>MQGSVTEFLKPRLVDIEQVSSTHAKVTLEPLERGFGHTLGNALRRILLSSMPGCAVTEVEIDGVLHEYSTKEGVQEDILEILLNLKGLAVRVQGKDEVILTLNKSGIGPVTAADITHDGDVEIVKPQHVICHLTDENASISMRIKVQRGRGYVPASTRIHSEEDERPIGRLLVDACYSPVERIAYNVEAARVEQRTDLDKLVIEMETNGTIDPEEAIRRAATILAEQLEAFVDLRDVRQPEVKEEKPEFDPILLRPVDDLELTVRSANCLKAEAIHYIGDLVQRTEVELLKTPNLGKKSLTEIKDVLASRGLSLGMRLENWPPASIADE[2x];> MVYSYTEKKRIRKDFGKRPQVLDVPYLLSIQLDSFQKFIEQDPEGQYGLEAAFRSVFPIQSYSGNSELQYVSYRLGEPVFDVQECQIRGVTYSAPLRVKLRLVIYEREAPEGTVKDIKEQEVYMGEIPLMTDNGTFVINGTERVIVSQLHRSPGVFFDSDKGKTHSSGKVLYNARIIPYRGSWLDFEFDPKDNLFVRIDRRRKLPATIILRALNYTTEQILDLFFEKVIFEIRDNKLQMELVPERLRGETASFDIEANGKVYVEKGRRITARHIRQLEKDDVKLIEVPVEYIAGKVVAKDYIDESTGELICAANMELSLDLLAKLSQSGHKRIETLFTNDLDHGPYISETLRVDPTNDRLSALVEIYRMMRPGEPPTREAAESLFENLFFSEDRYDLSAVGRMKFNRSLLREEIEGSGILSKDDIIDVMKKLIDIRNGKGEVDDIDHLGNRRIRSVGEMAENQFRVGLVRVERAVKERLSLGDLDTLMPQDMINAKPISAAVKEFFGSSQLSQFMDQNNPLSEITHKRRISALGPGGLTRERAGFEVRDVHPTHYGRVCPIETPEGPNIGLINSLSVYAQTNEYGFLETPYRKVTDGVVTDEIHYLSAIEEGNYVIAQANSNLDEEGHFVEDLVTCRSKGESSLFSRDQVDYMDVSTQQVVSVGASLIPFLEHDDANRALMGANMQRQAVPTLRADKPLVGTGMERAVAVDSGVTAVAKRGGVVQYVDASRIVIKVNEDEMYPGEAGIDIYNLTKYTRSNQNTCINQMPCVSLGEPVERGDVLADGPSTDLGELALGQNMRVAFMPWNGYNFEDSILVSERVVQEDRFTTIHIQELACVSRDTKLGPEEITADIPNVGEAALSKLDESGIVYIGAEVTGGDILVGKVTPKGETQLTPEEKLLRAIFGEKASDVKDSSLRVPNGVSGTVIDVQVFTRDGVEKDKRALEIEEMQLKQAKKDLSEELQILEAGLFSRIRAVLVAGGVEAEKLDKLPRDRWLELGLTDEEKQNQLEQLAEQYDELKHEFEKKLEAKRRKITQGDDLAPGVLKIVKVYLAVKRRIQPGDKMAGRHGNKGVISKINPIEDMPYDENGTPVDIVLNPLGVPSRMNIGQILETHLGMAAKGIGDKINAMLKQQQEVAKLREFIQRAYDLGADVRQKVDLSTFSDEEVMRLAENLRKGMPIATPVFDGAKEAEIKELLKLGDLPTSGQIRLYDGRTGEQFERPVTVGYMYMLKLNHLVDDKMHARSTGSYSLVTQQPLGGKAQFGGQRFGEMEVWALEAYGAAYTLQEMLTVKSDDVNGRTKMYKNIVDGNHQMEPGMPESFNVLLKEIRSLGINIELEDE;> MKDLLKFLKAQTKTEEFDAIKIALASPDMIRSWSFGEVKKPETINYRTFKPERDGLFCARIFGPVKDYECLCGKYKRLKHRGVICEKCGVEVTQTKVRRERMGHIELASPTAHIWFLKSLPSRIGLLLDMPLRDIERVLYFESYVVIEGGMTNLERQQILTEEQYLDALEEFGDEFDAKMGAEAIQALLKSMDLEQECEQLREELNETNSETKRKKLTKRIKLLEAFVQSGNKPEWMILTVLPVLPPDLRPLVPLDGGRFATSDLNDLYRRVINRNNRLKRLLDLAAPDIIVRNEKRMLQEAVDALLDNGRRGRAITGSNKRPLKSLADMIKGKQGRFRQNLLGKRVDYSGRSVITVGPYLRLHQCGLPKKMALELFKPFIYGKLELRGLATTIKAAKKMVEREEAVVWDILDEVIREHPVLLNRAPTLHRLGIQAFEPVLIEGKAIQLHPLVCAAYNADFDGDQMAVHVPLTLEAQLEARALMMSTNNILSPANGEPI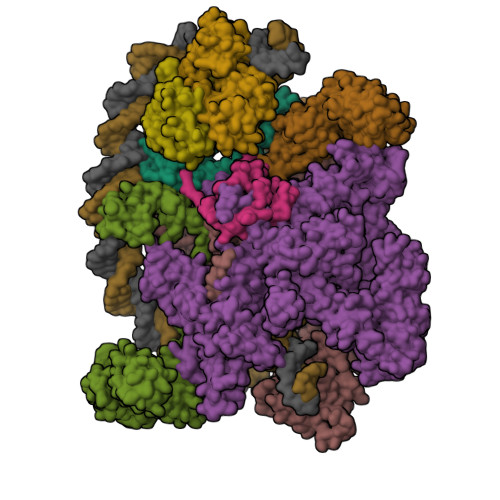IVPSQDVVLGLYYMTRDCVNAKGEGMVLTGPKEAERLYRSGLASLHARVKVRITEYEKDANGELVAKTSLKDTTVGRAILWMIVPKGLPYSIVNQALGKKAISKMLNTCYRILGLKPTVIFADQIMYTGFAYAARSGASVGIDDMVIPEKKHEIISEAEAEVAEIQEQFQSGLVTAGERYNKVIDIWAAANDRVSKAMMDNLQTETVINRDGQEEKQVSFNSIYMMADSGARGSAAQIRQLAGMRGLMAKPDGSIIETPITANFREGLNVLQYFISTHGARKGLADTALKTANSGYLTRRLVDVAQDLVVTEDDCGTHEGIMMTPVIEGGDVKEPLRDRVLGRVTAEDVLKPGTADILVPRNTLLHEQWCDLLEENSVDAVKVRSVVSCDTDFGVCAHCYGRDLARGHIINKGEAIGVIAAQSIGEPGTQLTMRTFHIGGAASRAAAESSIQVKNKGSIKLSNVKSVVNSSGKLVITSRNTELKLIDEFGRTKESYKVPYGAVLAKGDGEQVAGGETVANWDPHTMPVITEVSGFVRFTDMIDGQTITRQTDELTGLSSLVVLDSAERTAGGKDLRPALKIVDAQGNDVLIPGTDMPAQYFLPGKAIVQLEDGVQISSGDTLARIPQESGGTKDITGGLPRVADLFEARRPKEPAILAEISGIVSFGKETKGKRRLVITPVDGSDPYEEMIPKWRQLNVFEGERVERGDVISDGPEAPHDILRLRGVHAVTRYIVNEVQDVYRLQGVKINDKHIEVIVRQMLRKATIVNAGSSDFLEGEQVEYSRVKIANRELEANGKVGATYSRDLLGITKASLATESFISAASFQETTRVLTEAAVAGKRDELRGLKENVIVGRLIPAGTGYAYHQDRMRRRAAGEAPAAPQVTAEDASASLAELLNAGLGGSDNEHHHHHH;> ARVTVQDAVEKIGNRFDLVLVAARRARQMQVGGKDPLVPEENDKTTVIALREIEEGLINNQILDVRERQEQQEQEAAELQAVTAIAEGRR;> MEQNPQSQLKLLVTRGKEQGYLTYAEVNDHLPEDIVDSDQIEDIIQMINDMGIQVMEEAPDADDLMLAENTADEDAAEAAAQVLSSVESEIGRTTDPVRMYMREMGTVELLTREGEIDIAKRIEDGINQVQCSVAEYPEAITYLLEQYNRVEAEEARLSDLITGFVDPNAEEDLAPTATHVGSELSQEDLDDDEDEDEEDGDDDSADDDNSIDPELAREKFAELRAQYVVTRDTIKAKGRSHATAQEEILKLSEVFKQFRLVPKQFDYLVNSMRVMMDRVRTQERLIMKLCVEQCKMPKKNFITLFTGNETSDTWFNAAIAMNKPWSEKLHDVSEEVHRALQKLQQIEEETGLTIEQVKDINRRMSIGEAKARRAKKEMVEANLRLVISIAKKYTNRGLQFLDLIQEGNIGLMKAVDKFEYRRGYKFSTYATWWIRQAITRSIADQARTIRIPVHMIETINKLNRISRQMLQEMGREPTPEELAERMLMPEDKIRKVLKIAKEPISMETPIGDDEDSHLGDFIEDTTLELPLDSATTESLRAATHDVLAGLTAREAKVLRMRFGIDMNTDHTLEEVGKQFDVTRERIRQIEAKALRKLRHPSRSEVLRSFLDD;>[2x]VLGKPQTDPTLEWFLSHCHIHKYPSKSTLIHQGEKAETLYYIVKGSVAVLIKDEEGKEMILSYLNQGDFIGELGLFEEGQERSAWVRAKTACEVAEISYKKFRQLIQVNPDILMRLSAQMARRLQVTSEKVGNLAFLDVTGRIAQTLLNLAKQPDAMTHPDGMQIKITRQEIGQIVGCSRETVGRILKMLEDQNLISAHGKTIVVYGTR> MVLRDKMILLDENTKAIVQGITGRQGSFHTKKMLECGTKIVGGVTPGKGGQNVHGVPVFDTVKEAVKETDANASVIFVPAPFAKDAVFEAIDAGIELIVVITEHIPVHDTMEFVNYAEDVGVKIIGPNTPGIASPKVGKLGIIPMEVLKEGSVGMVSRSGTLTYEIAHQIKKAGFGVSTCVGIGGDPIVGLRYKEVLDLFEKDDETEAIVMIGEIGGGAEEEAAKFIEK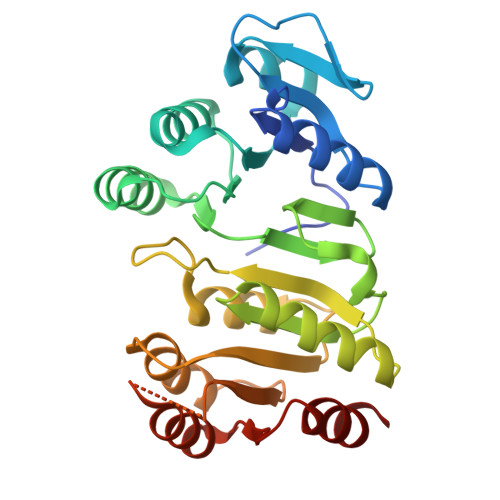MKKPVIGYIAGQSAPEGKRMGHAGAIVEKGKGTAESKMKALEEAGAYVAKNISDIPKLLAGILGK>[2x]GTPLVSEEELKLILAGAEESGAIQPQEEEMIHSILELEETPVREIMTPRVEMVAIEDEATLEDLLALYREHRYSRVPVYRESVDHIVGVAYAKDLLDYYAE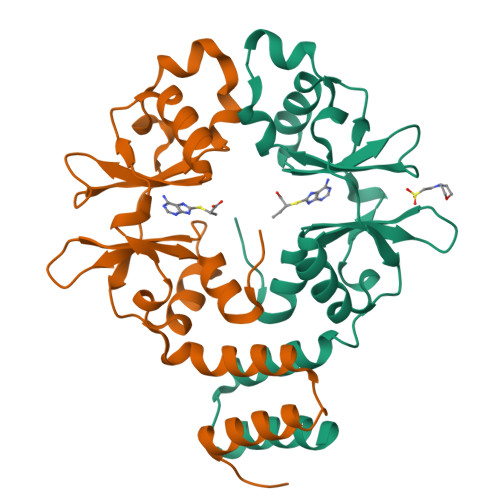EDLKGRTVASITHPPYFVPENMDAWSLLKELRRRKVHMAIVVDEFGGTAGLVILEDVIEEIVGEIYDETDEPEDAAIR>MAKKNKMKPRELREAQKKARQLKAAEINNNAAPAIAAMPAAEVIAPVAEKKKSSVKAAGMKSILVSENKMYITSFGKGNSAVLEYEVDNNDYNKTQLSSKDNSNIELGDVNEVNITFSSKHGFGSGVEINTSNPTHRSGESSPVRGDMLGLKSELEKRFFGKTFDDNIHIQLIYNILDIEKILAVYVTNIVYALNNMLGIKDSESYDDFMGYLSARNTYEVFTHPDKSNLSDKVKGNIKKSLSKFNDLLKTKRLGYFGLEEPKTKDTRASEAYKKRVYHMLAIVGQIAQCVFHDKSGAKRFDLYSFINNIDPEYRDTLDYLVEERLKSINKDFIEGNKVNISLLIDMMKGYEADDIIRLYYDFIVLKSQKNLGFSIKKLREKMLEEYGFRFKDKQYDSVRSKMYKLMDFLLFCNYYRNDVAAGEALVRKLRFSMTDDEKEGIYADEAAKLWGKFRNDFENIADHMNGDVIKELGKADMDFDEKILDSEKKNASDLLYFSKMIYMLTYFLDGKEINDLLTTLISKFDNIKEFLKIMKSSAVDVECELTAGYKLFNDSQRITNELFIVKNIASMRKPAASAKLTMFRDALTILGIDDNITDDRISEILKLKEKGKGIHGLRNFITNNVIESSRFVYLIKYANAQKIREVAKNEKVVMFVLGGIPDTQIERYYKSCVEFPDMNSSLEAKRSELARMIKNISFDDFKNVKQQAKGRENVAKERAKAVIGLYLTVMYLLVKNLVNVNARYVIAIHCLERDFGLYKEIIPELASKNLKNDYRILSQTLCELCDDRNESSNLFLKKNKRLRKCVEVDINNADS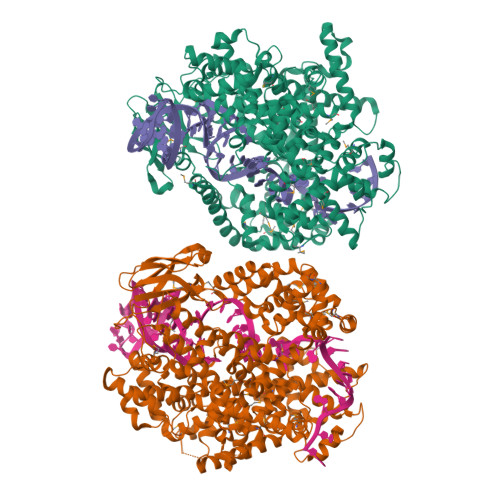SMTRKYANCIAHLTVVRELKEYIGDIRTVDSYFSIYHYVMQRCITKRGDDTKQEEKIKYEDDLLKNHGYTKDFVKALNSPFGYNIPRFKNLSIEQLFDRNEYLTEKLEHHHHHH[2x]>[2x]DYFQGAMGSKPAYSFHVTADGQMQPVPFPPDALIGPGIPRHARQINTLNHGEVVCAVTISNPTRHVYTGGKGCVKVWDISHPGNKSPVSQLDCLNRDNYIRSCKLLPDGCTLIVGGEASTLSIWDLAAPTPRIKAELT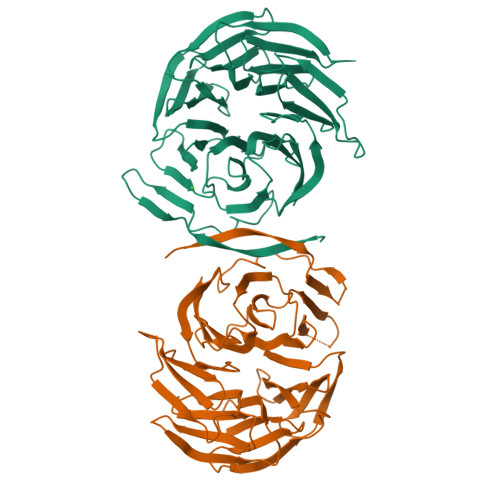SSAPACYALAISPDSKVCFSCCSDGNIAVWDLHNQTLVRQFQGHTDGASCIDISNDGTKLWTGGLDNTVRSWDLREGRQLQQHDFTSQIFSLGYCPTGEWLAVGMESSNVEVLHVNKPDKYQLHLHESCVLSLKFAYCGKWFVSTGKDNLLNAWRTPYGASIFQSKESSSVLSCDISVDDKYIVTGSGDKKATVYEVIY> AAPAYGQPSAAMGQNMRPMNQLYPIDLLTELPPPITDLTLPPPPLVIPPERMLVPSELSNASPDYIRSTLNAVPKNSSLLKKSKLPFGLVIRPYQHLYDDIDPPPLNEDGLIVRCRRCRSYMNPFVTFIEQGRRWRCNFCRLANDVPMQMDQSDPNDPKSRYDRNEIKCAVMEYMAPKEYTLRQPPPATYCFLIDVSQSSIKSGLLATTINTLLQNLDSIPNHDERTRISILCVDNAIHYFKIPLDSENNEESADQINMMDIADLEEPFLPRPNSMVVSLKACRQNIETLLTKIPQIFQSNLITNFALGPALKSAYHLIGGVGGKIIVVSGTLPNLGIGKLQRRNESGVVNTSKETAQLLSCQDSFYKNFTIDCSKVQITVDLFLASEDYMDVASLSNLSRFTAGQTHFYPGFSGKNPNDIVKFSTEFAKHISMDFCMETVMRARGSTGLRMSRFYGHFFNRSSDLCAFSTMPRDQSYLFEVNVDESIMADYCYVQVAVLLSLNNSQRRIRIITLAMPTTESLAEVYASADQLAIASFYNSKAVEKALNSSLDDARVLINKSVQDILATYKKEIVVSNTAGGAPLRLCANLRMFPLLMHSLTKHMAFRSGIVPSDHRASALNNLESLPLKYLIKNIYPDVYSLHDMADEAGLPVQTEDGEATGTIVLPQPINATSSLFERYGLYLIDNGNELFLWMGGDAVPALVFDVFGTQDIFDIPIGKQEIPVVENSEFNQRVRNIINQLRNHDDVITYQSLY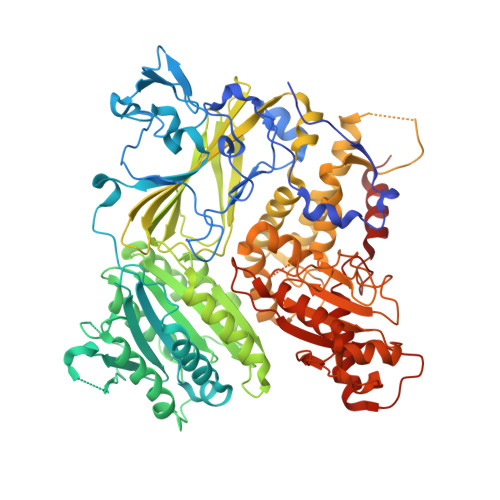IVRGASLSEPVNHASAREVATLRLWASSTLVEDKILNNESYREFLQIMKARISK>[6x]GSIAPYLVKIIDPDYEKNERTRIKAQENLRRIRRKQIAEKGDNEDGTDDPSRRRKIDDLVLNEYENQVALEVVAPEDIPVGFNDIGGLDDIIEELKETIIYPLTMPHLYKHGGALLAAPSGVLLYGPPGCGKTMLAKAVAHESGASFINLHISTLTEKWYGDSNKIVRAVFSLAKKLQPSIIFIDQIDAVLGTRRSGEHEASGMVKAEFMTLWDGLTSTNASGVPNRIVVLGATNRINDIDEAILRRMPKQFPVPLPGLEQRRRILELVLRGTKRDPDFDLDYIARVTAGMSGSDIKETCRDAAMAPMREYIRQHRASGKPLSEINPDDVRGIRTEDFFGRRGGKILSEIPPRQTGYVVQSKNSSEGGYEEVEDDDEQGTAST

The AAA protein Msp1 (in yeast; ATAD1 in mammals) extracts the tail-anchored (TA) membrane proteins that have failed to be correctly inserted into the ER membrane. TA proteins that escape this reaction are mistargeted to the mitochondrial outer membrane (MOM), necessitating their removal. This proofreading function is performed by Msp1/ATAD1, which extracts the mistargeted TA proteins from the MOM to facilitate their subsequent proteasomal degradation. Here, we present a collection of three high-resolution Msp1 solution-state structures (an ATP hydrolysis-arrested Msp1 mutant and two conformational states of wildtype Msp1) that address these outstanding questions and begin to explain how particular features, shared by AAAMC proteins adapt it to its particular roles in protein quality control and beyond. To obtain a homogeneous sample suitable for structural studies, we expressed the cytosolic domain of Msp1 lacking its 30 amino acid N-terminal membrane anchor (Δ30-Msp1) from the thermophilic yeast Chaetomium thermophilum.

In addition, we expressed and purified a mutant form of Δ30-Msp1, Δ30-Msp1E214Q, bearing a commonly used ‘Walker B’ mutation that inactivates ATP hydrolysis but leaves ATP binding intact. Δ30-Msp1 formed homogeneous hexamers as assessed by size-exclusion chromatography, whereas Δ30-Msp1E214Q formed hexamers but also higher order oligomers. We incubated Δ30-Msp1 with ADP•BeFx, an ATP transition state analog that in ATPases (depending on whether BeFx is bound) can mimic both the ATP and the ADP states, and Δ30-Msp1E214Q with ATP. 3D classification of Δ30-Msp1E214Q particles revealed two distinct structures. The structure closely resembles the open conformation of Δ30-Msp1 (RSMD = 0.867). Second, 38,165 particles contributed to a reconstruction of Msp1 showing extra density, indicative of the presence of one or more extra 30-Msp1E214Q subunits extending the spiral staircase (Figure 1—figure supplements 5B and 6). Henceforth, we focus our analyses exclusively on the structure of the homogeneous hexamer, because we observed the higher oligomers only in the context of the E214Q mutation. In Δ30-Msp1E214Q, M1-M5 display clear density for ATP, whereas M6 does not contain significant density for a nucleotide, again indicating that M6 is in a distinct conformation from the other subunits. The Δ30-Msp1E214Q structure serves as a convenient control: M5 in Δ30-Msp1E214Q binds to an ATP instead of ADP and the corresponding WD motif and NCL in M6 are both well-ordered, supporting our hypothesis that the NCL melts in response to ATP hydrolysis. Upon modeling the protein into the density, we observed in all three structures extra density in the central pore of the spiral, spanning its entire depth. This density likely represents an averaged composite of a mixture of peptides from endogenous E. coli proteins that engaged with and became trapped in the central translocation pore.>EFGSMEFVNKQFNYKDPVNGVDIAYIKIPNAGQMQPVKAFKIHNKIWVIPERDTFTNPEEGDLNPPPEAKQVPVSYYDSTYLSTDNEKDNYLKGVTKLFERIYSTDLGRMLLTSIVRGIPFWGGSTIDTELKVIDTNCINVIQPDGSYRSEELNLVIIGPSADIIQFECKSFGHEVLNLTRNGYGSTQYIRFSPDFTFGFEESLEVDTNPLLGAGKFATDPAVTLAHELIHAGHRLYGIAINPNRVFKVNTNAYYEMSGLEVSFEELRTFGGHDAKFIDSLQENEFRLYYYNKFKDIASTLNKAKSIVGTTASLQYMKNVFKEKYLLSEDTSGKFSVDKLKFDKLYKMLTEIYTEDNFVKFFKVLNRKTYLNFDKAVFKINIVPKVNYTIYDGFNLRNTNLAANFNGQNTEINNMNFTKLKNFTGLFEFYKLLCVDGIITSKTKSLIEGR[2x];>NKALNLQCIKVNNWDLFFSPSEDNFTNDLNKGEEITSDTNIEAAEENISLDLIQQYYLTFNFDNEPENISIENLSSDIIGQLELMPNIERFPNGKKYELDKYTMFHYLRAQEFEHGKSRIAL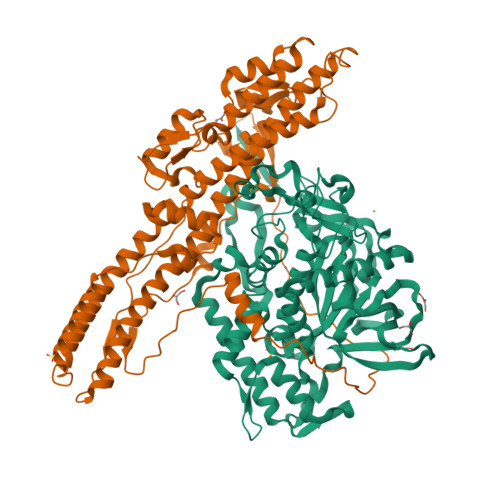TNSVNEALLNPSRVYTFFSSDYVKKVNKATEAAMFLGWVEQLVYDFTDETSEVSTTDKIADITIIIPYIGPALNIGNMLYKDDFVGALIFSGAVILLEFIPEIAIPVLGTFALVSYIANKVLTVQTIDNALSKRNEKWDEVYKYIVTNWLAKVNTQIDLIRKKMKEALENQAEATKAIINYQYNQYTEEEKNNINFNIDDLSSKLNESINKAMININKFLNQCSVSYLMNSMIPYGVKRLEDFDASLKDALLKYIYDNRGTLIGQVDRLKDKVNNTLSTDIPFQLSKYVDNQRLLSTFTEYIKNIINTS[2x]> VVGGLVALRGAHPYIAALYWGHSFCAGSLIAPCWVLTAAHCLQDRPAPEDLTVVLGQERRNHSCEPCQTLAVRSYRLHEAFSPVSYQHDLALLRLQEDADGSCALLSPY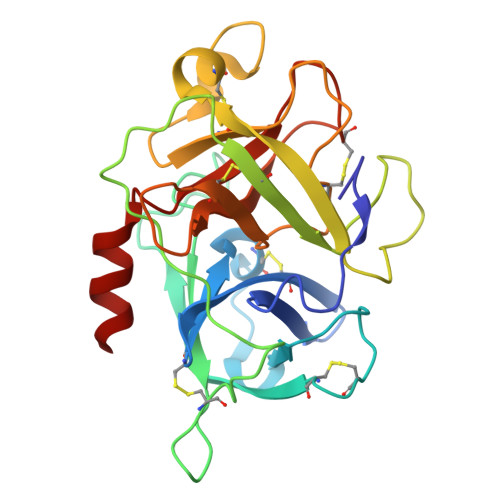VQPVCLPSGAARPSETTLCQVAGWGHQFEGAEEYASFLQEAQVPFLSLERCSAPDVHGSSILPGMLCAGFLEGGTDACQGDSGGPLVCEDQAAERRLTLQGIISWGSGCGDRNKPGVYTDVAYYLAWIREHTVS>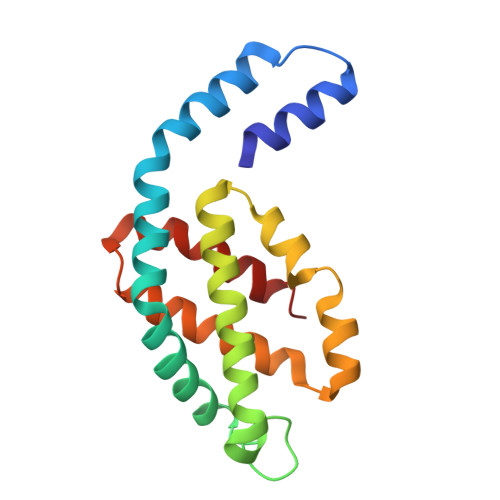 MSVVTKSIVNADAEARYLSPGELDRIKNFVSTGERRLRIAQTLTENRERIVKQAGDQLFQKRPDVVSPGGNAYGEEMTATCLRDLDYYLRLVTYGIVAGDVTPIEEIGLVGVREMYNSLGTPIPAVAEGIRAMKNVACSLLSAEDAAEAGSYFDFVIGAMQ> GSSPEKPTPNGGIPHDNLVLIRMKPDENGRFGFNVKGGYDQKMPVIVSRVAPGTPADLCVPRLNEGDQVVLINGRDIAEHTHDQVVLFIKASCERHSGELML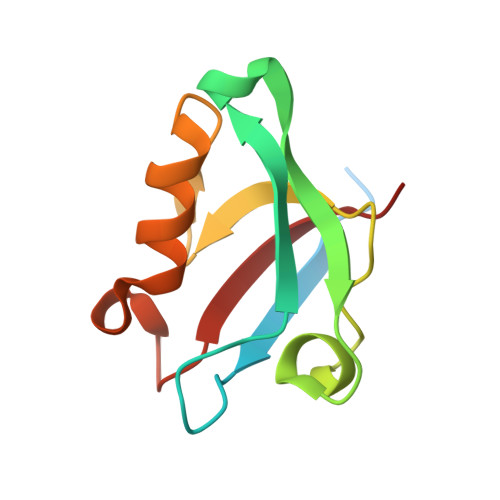LVRPN> GSTKETAFVEVVLFESSPSGDYTTYTTGLTGRF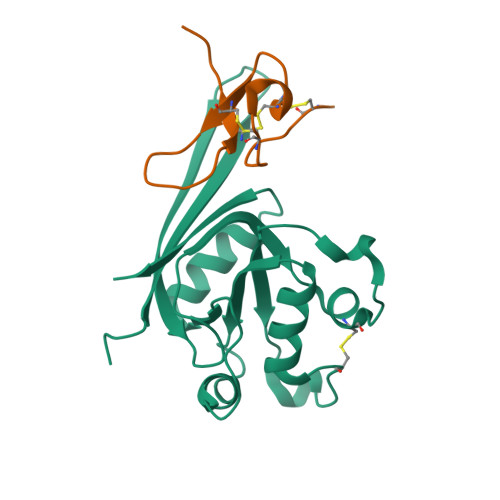SRAGATLSAEGEIVQMHPLGLCNNNDEEDLYEYGWVGVVKLEQPELDPKPCLTVLGKAKRAVQRGATAVIFDVSENPEAIDQLNQGSEDPLKRPVVYVKGADAIKLMNIVNKQKVARARIQHRPPRQPTEYFDMGNSDYKDDDDK;> GCNRLNKKCNSDADCCANKEKCERPIGWKFMYCRPDVGP>[2x]GAMAHAAALSVR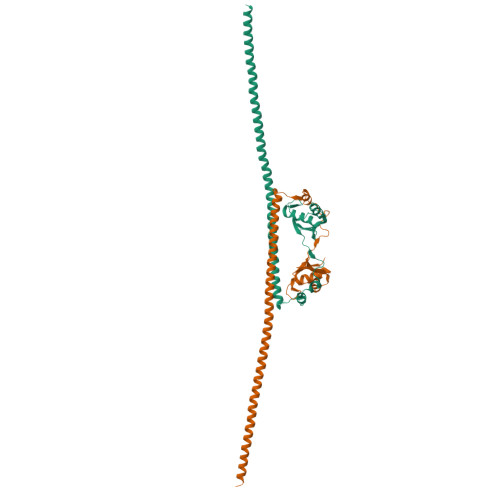NLSPYVSNELLEEAFSQFGPIERAVVIVDDRGRSTGKGIVEFASKPAARKAFERCSEGVFLLTTTPRPVIVEPLEQLDDEDGLPEKLAQKNPMYQKERETPPRFAQHGTFEYEYSQRWKSLDEMEKQQREQVEKNMKDAKDKLESEMEDAYHEHQANLLRQDLMRRQEELRRMEELHNQEMQKRKEMQLRQEEERRRREEEMMIRQREMEEQMRRQREESYS> MTDTTNSIKHVISPLARQTLQDRDLTRPVAGKRPIRLLPWLQVVKIGGRVMDRGADAILPLVEELRKLLPEHRLLILTGAGVRARHVFSVGLDLGLPVGSLAPLAASEAGQNGHILA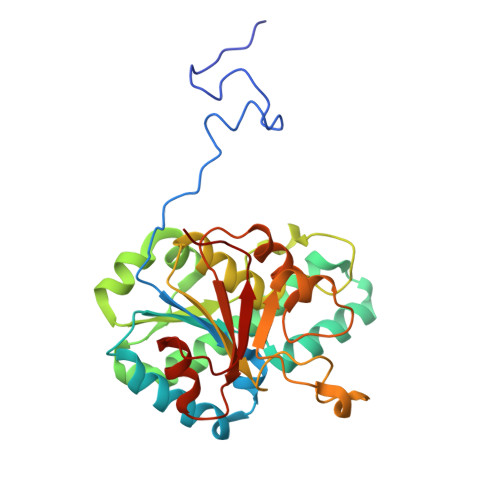AMLASEGVSYVEHPTVADQLAIHLSATRAVVGSAFPPYHHHEFPGSRIPPHRADTGAFLLADAFGAAGLTIVENVDGIYTADPNGPDRGQARFLPETSATDLAKSEGPLPVDRALLDVMATARHIERVQVVNGLVPGRLTAALRGEHVGTLIRTGVRPA>[3x]MGHKLAFNFNLEINGSDTHSTVDVYLDDSQIITFDGKDIRPTIPFMIGDEIFLPFYKNVFSEFFSLFRRVPTSTPYEDLTYFYECDYTDNKSTFDQFYLYNGEEYTVKTQEA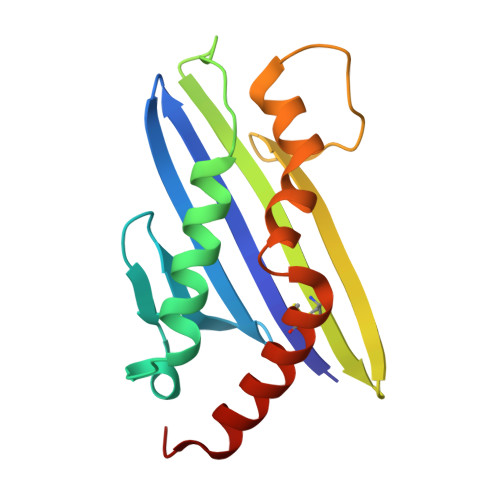TNKNMWLTTSEFRLKKWFDGEDCIMHLRSLVRKMEDSKR1-methylindol-5-amine | C9 H10 N2 | 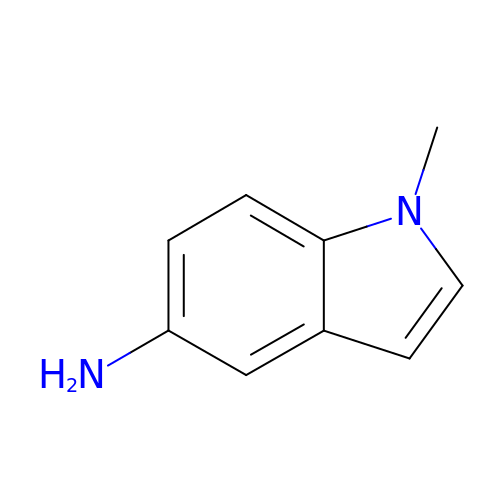PGTSGPCXPIFQEL-UHFFFAOYSA-N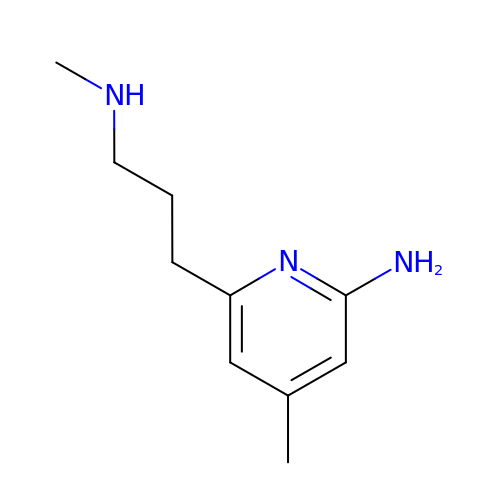4-methyl-6-[3-(methylamino)propyl]pyridin-2-amine | C10 H17 N3 | MOHLCKRYTZYOGZ-UHFFFAOYSA-N> APKAP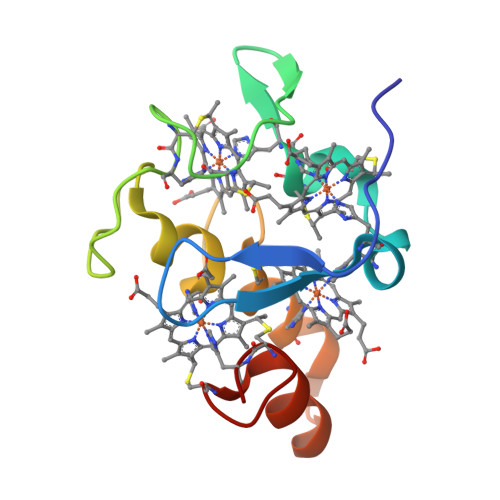ADGLKMDKTKQPVVMNHSTHKAVKCGDCHHPVNGKEDYQKCATAGCHDNMDKKDKSAKGYYHAMHDKGTKFKSCVGCHLETAGADAAKKKELTGCKGSKCHS>[3x]MKKILDSA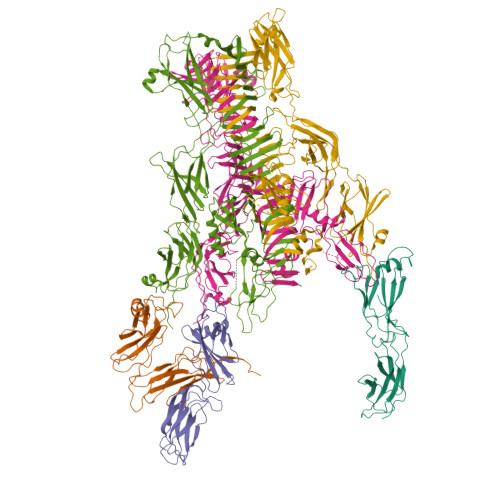KNYLNTHDKLKTACLIALELPSSSGSAATYIYLTDYFRDVTYNGILYRSGKVKSISSHKQNRQLSIGSLSFTITGTAEDEVLKLVQNGVSFLDRGITIHQAIINEEGNILPVDPDTDGPLLFFRGRITGGGIKDNVNTSGIGTSVITWNCSNQFYDFDRVNGRYTDDASHRGLEVVNGTLQPSNGAKRPEYQEDYGFFHSNKSTTILAKYQVKEERYKLQSKKKLFGLSRSYSLKKYYETVTKEVDLDFNLAAKFIPVVYGVQKIPGIPIFADTELNNPNIVYVVYAFAEGEIDGFLDFYIGDSPMICFDETDSDTRTCFGRKKIVGDTMHRLAAGTSTSQPSVHGQEYKYNDGNGDIRIWTFHGKPDQTAAQVLVDIAKKKGFYLQNQNGNGPEYWDSRYKLLDTAYAIVRFTINENRTEIPEISAEVQGKKVKVYNSDGTIKADKTSLNGIWQLMDYLTSDRYGADITLDQFPLQKVISEAKILDIIDESYQTSWQPYWRYVGWNDPLSENRQIVQLNTILDTSESVFKNVQGILESFGGAINNLSGEYRITVEKYSTNPLRINFLDTYGDLDLSDTTGRNKFNSVQASLVDPALSWKTNSITFYNSKFKEQDKGLDKKLQLSFANITNYYTARSYADRELKKSRYSRTLSFSVPYKFIGIEPNDPIAFTYERYGWKDKFFLVDEVENTRDGKINLVLQEYGEDVFINSEQVDNSGNDIPDISNNVLPPRDFKYTPTPGGVVGAIGKNGELSWLPSLTNNVVYYSIAHSGHVNPYIVQQLENNPNERMIQEIIGEPAGLAIFELRAVDINGRRSSPVTLSVDLNSAKNLSVVSNFRVVNTASGDVTEFVGPDVKLAWDKIPEEEIIPEIYYTLEIYDSQDRMLRSVRIEDVYTYDYLLTYNKADFALLNSGALGINRKLRFRIRAEGENGEQSVGWATI;>[3x]MISNNAPAKMVLNSVLTGYTLAYIQHSIYSDYDVIGRSFWLKEGSNVTRRDFTGIDTFSVTINNLKPTTTYEVQGAFYDSIIDSELLNAQIGINLSDKQTFKMKSAPRITGARCESEPVDVGVGAPIVYIDTTGEADYCTIELKDNSNANNPWVKYYVGALMPTIMFGGVPIGSYKVRISGQISLPDGVTIDSSGYYEYPNVFEVRYNFVPPAAPINIVFKAARIADGKERYDLRVQWDWNRGAGANVREFVLSYIDSAEFVRTGWTKAQKINVGAAQSATIISFPWKVEHKFKVSSIAWGPDAQDVTDSAVQTFILNESTPLDNSFVNETGIEVNYAYIKGKIKDGSTWKQTFLIDAATGAINIGLLDAEGKAPISFDPVKKIVNVDGSVITKTINAANFVMTNLTGQDNPAIYTQGKTWGDTKSGIWMGMDNVTAKPKLDIGNATQYIRYDGNILRISSEVVIGTPNGDIDIQTGIQGKQTVFIYIIGTSLPAKPTSPAYPPSGWSKTPPNRTSNTQNIYCSTGTLDPVTNQLVSGTSWSDVVQWSGTEGVDGRPGATGQRGPGMYSLAIANLTAWNDSQANSFFTSNFGSGPVKYDVLTEYKSGAPGTAFTRQWNGSAWTSPAMVLHGDMIVNGTVTASKIVANNAFLSQIGVNIIYDRAAALSSNPEGSYKMKIDLQNGYIHIR>[2x]SPDKLKKVLDKLRLDPKDISEAAETVNKVVERLLRRMQKRESEFKGVEQLLVGSFYEKVKISAPNEFDVMFKLEVPRIELQEYYETGAFYLVKFKRIPRGNPLSHFLEGEVLSATKMLSKFRKIIKEEVKEIKD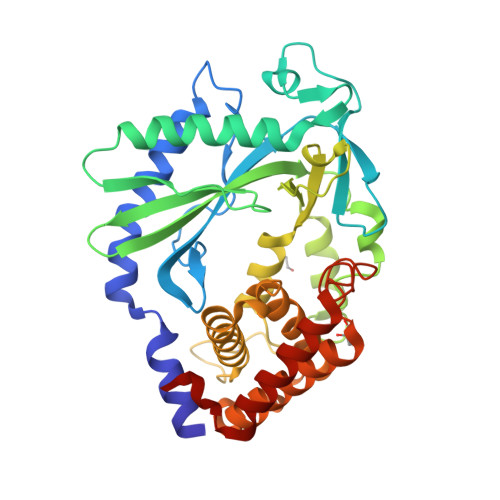IDVSVEKEKPGSPAVTLLIRNPEEISVDIILALESKGSWPISTKEGLPIQGWLGTKVRTNLRREPFYLVPKNAKDGNSFQGETWRLSFSHTEKYILNNHGIEKTCCESSGAKCCRMECLMLMKYLLEQLKKEFQELDAFCSYHVKTAIFHMWTQDPQDSQWDPRNLSSCFDKLLAFFLECLRTEKLDHYFIPKFNLFSQELIDRKSKEFLSKKIEYERNNGFPIFDKL>MGSSHHHHHHSMDNKTETKIEPKTGTTNFDQEALLYHQQGKPGKIEVISSKPCATEKDLSLAYSPGVAAPCKAIAKDPAKVYDYTAKGNLVAVISNGTAVLGLGNIGPAAGKPVMEGKGILFKQFAGIDVFDIEVAATDVDVFCNAVRVLEPTFGGINLEDIKAPECFEIEERLKKEMNIPVFHDDQHGTAI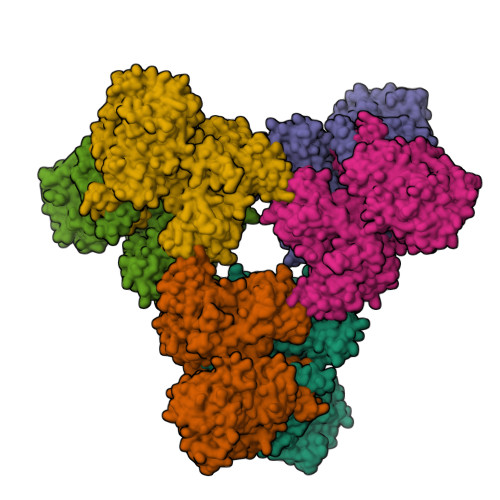VSGAALLNACSITNRKMETVRIVVNGAGASANSCAKIFIALGARRENIIMCDSQGVIYKGRTAGMNKYKEYFASETEARTLTEALRGADVFVGLSVAGALTPEMLKDMAKDPIIFAMANPEPEITPDKARAARPDAIIATGRSDYPNQVNNVLGFPSIFRGALDTRSTQINEEMKLAAVHALAKLAREDVPDKVSATYGGKSFKFGRDYLIPKPFDTRVLLWVAPEVAKAAMKSGVATRAIEDWDQYRESLEALQGPSKVFIRSAINRVHQNSAANGGELPRIVFPEGTSTKVLKALATLVEEKICQPILLGYPERVKEKIKALDIPLLNDVSIVHPSSHPKYFSFVEKLYSLRQRKGINLGEAERLMADPNYFAAMMVNQGEADGMVSGSSINYADAVRPILQTIGVYKEGIPAGLNFVLLEDKFLVLADTTVNLNPTAEQCAQIALQAAKIVEYFGIEPRVAMLSYSNFSGAEGTPRKMKKAAEIARSLRPDLMIEGDMQADTAVNPEIMERLFPFSGLKGGANVLVFPNLESSNIAYKLIQQIGKAEVIGPFLTGVRRSANVLQRTTTVDGIVNSVVFTALEAQYIKEVLKSRGKK[6x]>[2x]SPPRGKTVWFTGLSGSGKSSVAMLVERKLLEKGISAYVLDG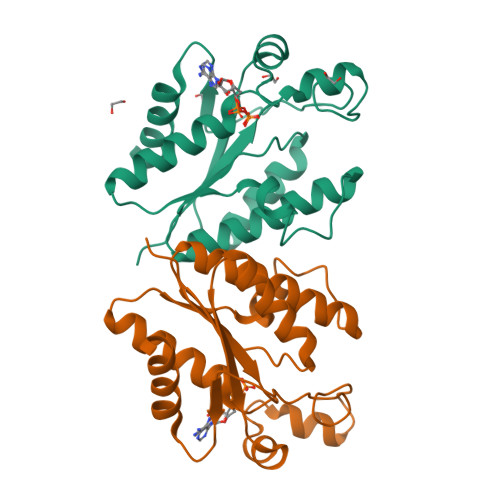DNLRHGLNADLGFSMADRAENLRRLSHVATLLADCGHLVLVPAISPLAEHRALARKVHADAGIDFFEVFCDTPLQDCERRDPKGLYAKARAGEITHFTGIDSPYQRPKNPDLRLTPDRSIDEQAQEVIDLLES> SNALSRYEKWEKIKQHYQHWSDSLSEEGRGLLKKLQIPIEPKKDDIIHSLSQEEKELLKRIQIDSSDFLSTEEKEFLKKLQIDIRDSLSEEEKELLNRIQVDSSNPLSEKEKEFLKKLKLDIQPYDINQRLQDTGGLIDSPSINLDVRKQYKRDIQNIDALLHQSIGSTLYNKIYLYENMNINNLTATLGADLVDSTDNTKINRGIFNEFKKNFKYSISSNYMIVDINERPALDNERLKWRIQL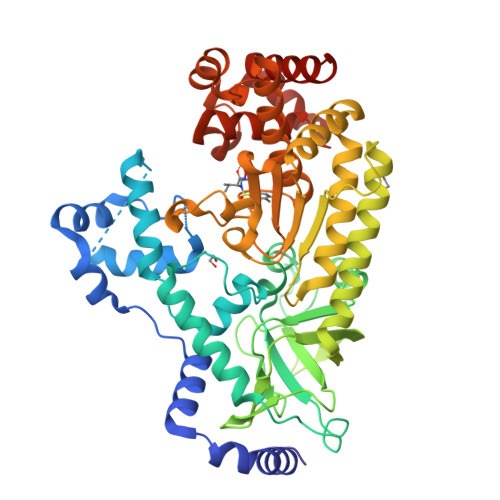SPDTRAGYLENGKLILQRNIGLEIKDVQIIKQSEKEYIRIDAKVVPKSKIDTKIQEAQLNINQEWNKALGLPKYTKLITFNVHNRYASNIVESAYLILNEWKNNIQSDLIKKVTNYLVDGNGRFVFTDITLPNIAEQYTHQDEIYEQVHSKGLYVPESRSILLHGPSKGVELRNDSEGFIHEFGHAVDDYAGYLLDKNQSDLVTNSKKFIDIFKEEGSNLTSYGRTNEAEFFAEAFRLMHSTDHAERLKVQKNAPKTFQFINDQIKFIINSLVPR7-METHYL-GUANOSINE-5'-TRIPHOSPHATE-5'-GUANOSINE | C21 H30 N10 O18 P3 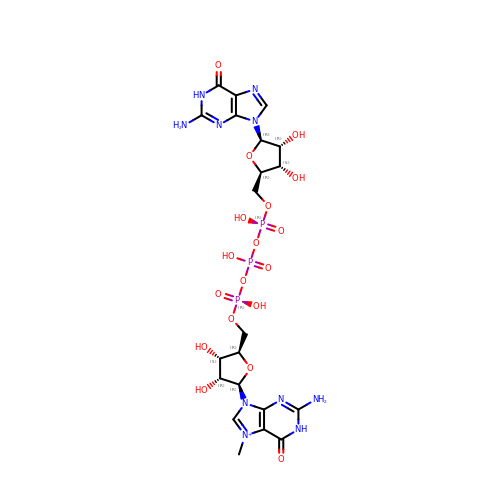| FHHZHGZBHYYWTG-INFSMZHSSA-O> MSAVKAARYGKDNVRVYKVHKDEKTGVQTVYEMTVCVLLEGEIETSYTKADNSVIVATDSIKNTIYITAKQNPVTPPELFGSILGTHFIEKYNHIHAAHVNIVCHRWTRMDIDGKPHPHSFIRDSEEKRNVQVDVVEGKGIDIKSSLSGLTVLKSTNSQFWGFLRDEYTTLKETWDRILSTDVDATWQWKNFSGLQEVRSHVPKFDATWATAREVTLKTFAEDNSASVQ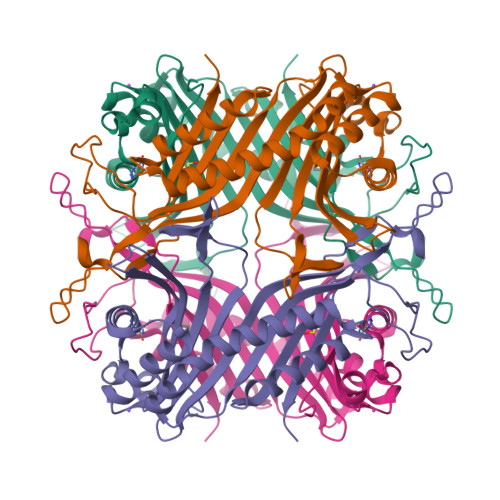ATMYKMAEQILARQQLIETVEYSLPNKHYFEIDLSWHKGLQNTGKNAEVFAPQSDPNGLIKCTVGRSSLKSKL>[6x]GSPSSTMGQVGRQLAIIGDDIN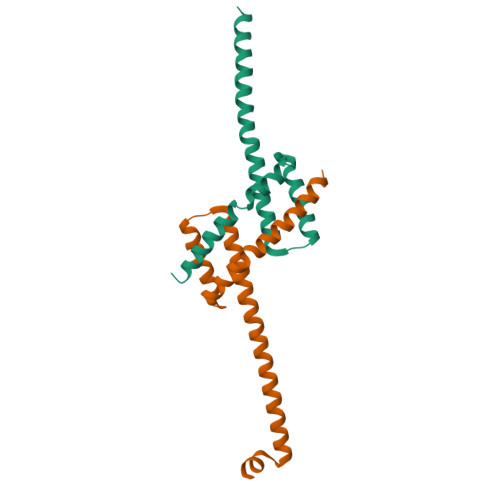RRYDSEFQTMLQHLQPTAENAYEYFTKIATSLFESGINWGRVVALLGFGYRLALHVYQHGLTGFLGQVTRFVVDFMLHHSIARWIAQRGGWVAALNLGNG> HEDSDKDHSFLTNDELAVLPVVKVLPSGKYTGANLKSVIRVLRGLLDQGIPSKELENLQELKPLDQCLIGQTKENRRKNRYKNILPYDATRVPLGDEGGYINASFIKI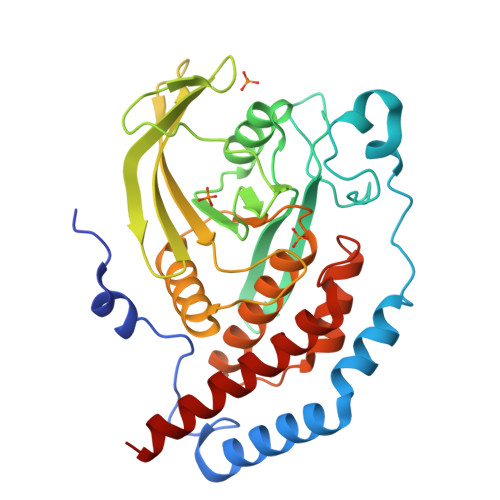PVGKEEFVYIACQGPLPTTVGDFWQMIWEQKSTVIAMMTQEVEGEKIKCQRYWPNILGKTTMVSNRLRLALVRMQQLKGFVVRAMTLEDIQTREVRHISHLNFTAWPDHDTPSQPDDLLTFISYMRHIHRSGPIITHCSAGIGRSGTLICIDVVLGLISQDLDFDISDLVRCMRLQRHGMVQTEDQYIFCYQVILYVLTRLQAEEEQ>[4x]MSELSVATGAVSTASSSIPMPAGVNPADLAAELAAVVTESVDEDYLLYECDGQWVLAAGVQAMVELDSDELRVIRDGVTRRQQWSGRPGAALGEAVDRLLLETDQAFGWVAF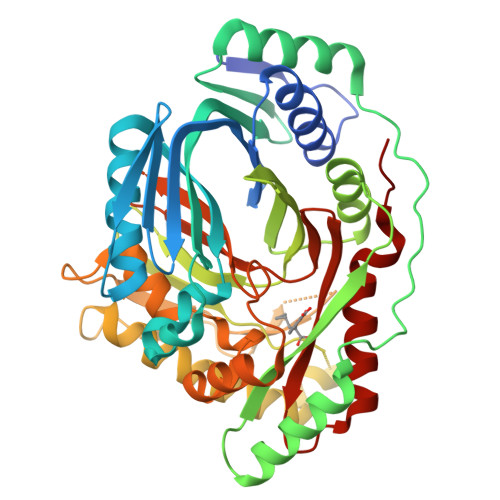EFGVHRYGLQQRLAPHTPLARVFSPRTRIMVSEKEIRLFDAGIRHREAIDRLLATGVREVPQSRSVDVSDDPSGFRRRVAVAVDEIAAGRYHKVILSRCVEVPFAIDFPLTYRLGRRHNTPVRSFLLQLGGIRALGYSPELVTAVRADGVVITEPLAGTRALGRGPAIDRLARDDLESNSKEIVEHAISVRSSLEEITDIAEPGSAAVIDFMTVRERGSVQHLGSTIRARLDPSSDRMAALEALFPAVTASGIPKAAGVEAIFRLDECPRGLYSGAVVMLSADGGLDAALTLRAAYQVGGRTWLRAGAGIIEESEPEREFEETCEKLSTLTPYLVARQ> MALPLPHQRLRLDPVPEFEELQKAGPLHEYDTEPGMDGRKQWLVTGHDEVRAILADHERFSSMRPVDDEADRALLPGILQAYDPPDHTRLRRTVAPAYSARRMERLRPRIEEIVEECLDDFESVGAPVDFVRHAAWPIPAYIACEFLGVPRDDQAELSRMIRESRESRLPRQRTLSGLGIVNYTKRLTSGKRRDPGDGMIGVIVREHGAEISDEELAGLAEGNLIMAAEQMAAQLAVAVLLLVTHPDQMALLREKPELIDSATEEVLRHASIVEAPAPRVALADVRMAGRDIHAGDVL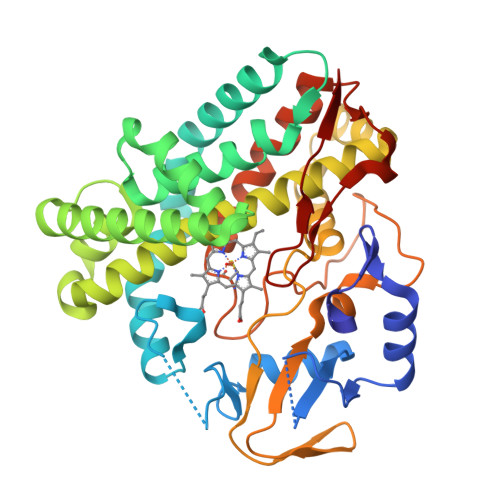TCSMLATNRAPGDRFDITREKATHMAFGHGIHHCIGAPLARLQLRVALPAVVGRFPSLRLAVPEEDLRFKPGRPAPFAVEELPLEW>[2x]SNAMDEGISKKFAIQLLEDDAERIKMLIR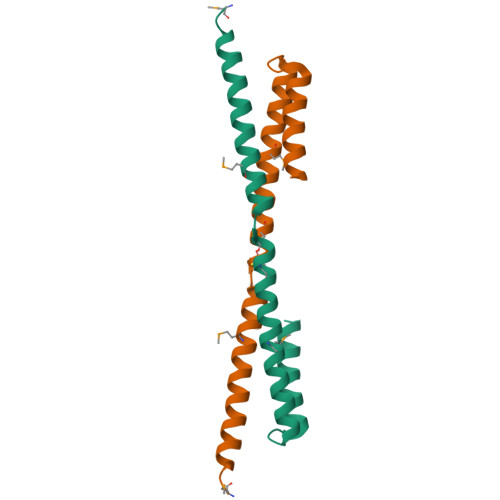NQKNSLCISQCKAFEEVVDTQMYGFSRQVTYATRLGILTNDEGHRLLSDLERELNQLYTDVYEETQEKNEIGKEG N-(3-PHENYL-2-SULFANYLPROPANOYL)PHENYLALANYLALANINE | C21 H24 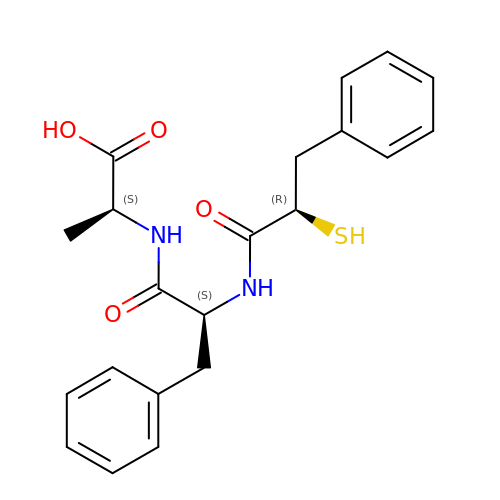N2 O4 S | CNILVMARPONFBX-JCGIZDLHSA-N> VTTTATLTYPFHDWSQELSPRYAQLRASDAPVCPVVSEGTGDPLWLVTRYATAVKLLEDSRFSSEAAQASGAPRQEPVELRAPGTRGDAIAMLREAGLRSVLADGLGPRAVRRHQGWINDLAETLMSELASREGTFDLAADFVEPLSSALVSRTLLGELSADERDLLAHCADTGLRFCGVTHEEQVHAFTQMHEFFLEHARRLAGTPGEHLLKLIAEAPVDQGPLSDEALAEAGSLLVVAGFPTSSGFLCGALLTLLRHPDAVQELHAHPERVPSAVEELLRYTPLSTGSVKRMATEDLEID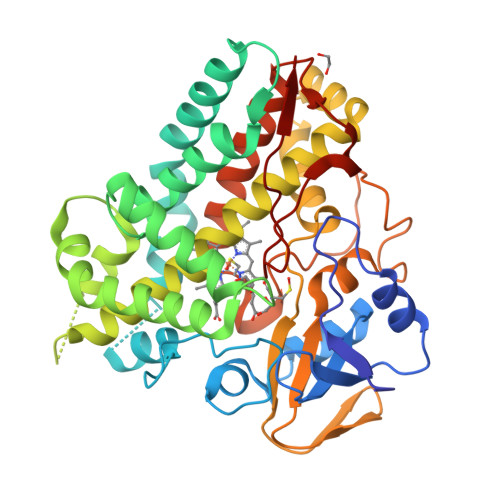GVRIKAGEVVMVSLEAVNHDPDAFEDPDVFRPGREGPMHFGFGRGRHFCPGNRLARCVIEATVRAVARRPGLRLAVAPEEISWHEGLFFRRPRAIPATW>SNADEDDSADNIHAVSSERWRIHAATEIEDINTFFGTEYSSEEADTIGGLVIQELGHLPVRGEKVLIGGLQFTVARADNRR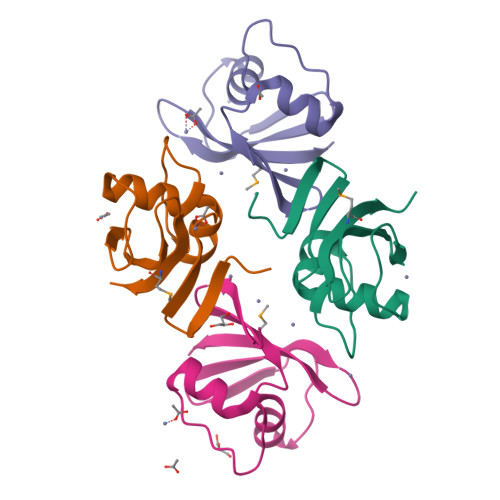LHTLMATRVK[4x]>[2x]METDLNSQDRKDLDKFIKFFALKTVQVIVQARLGEKICTRSSSSPTGSDWFNLAIKDIPEVTHEAKKALAGQLPAVGRSMCVEISLKTSEGDSMELEIWCLEMNEKCDKEIKVSYTVYNRLSLLLKSLLAITRVTPAYRLSRKQ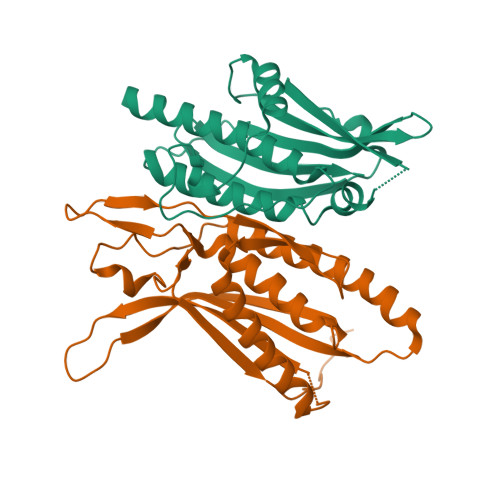GHEYVILYRIYFGEVQLSGLGEGFQTVRVGTVGTPVGTITLSCAYR;>MNCRSEVLEVSVEGRQVEEAMLAVLHTVLLHRSTGKFHYAAAGTYSIGTVGTQDVDCDFIDFTYVRVSSEELDRALRKVVGEFKDALRNSGGDGLGQMSLEFYQKKKSRWPFSDECIPWEVWTVKVHVVALATEQERQICREKVGEKLCEKIINIVEVMNRHEYLPKMPTQSEVDNVFDTGLRDVQPYLYKISFQITDALGTSVTTTMRRLIKDTLAL[2x]> MDETGKELVLVLYDYQE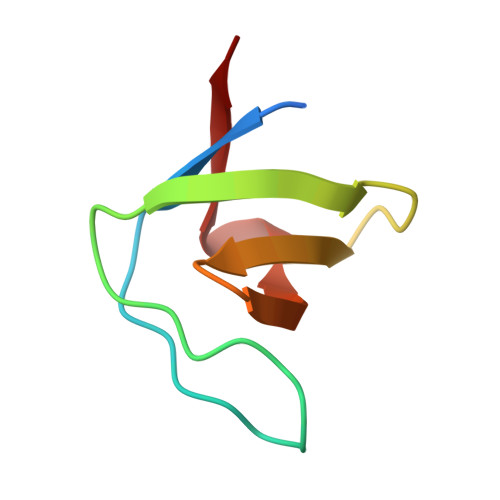KSPREVTVKKGDILTLLNSTNKDWWKVEVDDRQGFIPAAYLKKLD> MAFHWCDNNLHTTVFTPRDFQVELLATAYERNTIICLGHRSSKEFIALKLLQELSRRARRHGRVSVYLSCEVGTSTEPCSIYTMLTHLTDLRVWQEQPDMQIPFDHCWTDYHVSILRPEGFLYLLETRELLLSRVELIVLEDCHDSAVYQRIRPLFENHIMPAPPADRPRILGLAGPLHSAGCELQQLSAMLATLEQSVLCQIESASDIVTVLRYCSRPHEYIVQCAPFEMDELSLVLADVLNTHKSFLLDHRYDPYEIYGTDQFMDELKDIPDPKVDPLNVINSLLVVLHEMGPWCTQRAAHHFYQCNEKLKVKTPHERHYLLYCLVSTALIQLYSLCEHAFHRHLGSGSDSRQTIERYSSPKVRRLLQTLRCFKPEEVHTQADGLRRMRHQVDQADFNRLSHTLESKCRMVDQLDQPPTETRALVATLEQILHTTEDRQTNRSAARVTPTPTPAHAKPKPSSGANTAQPRTRRRVYTRRHHRDHNDGSDTLCALIYCNQNHTARVLFELLAEISRRDPDLKFLRCQYTTDRVADPTTEPKEAEL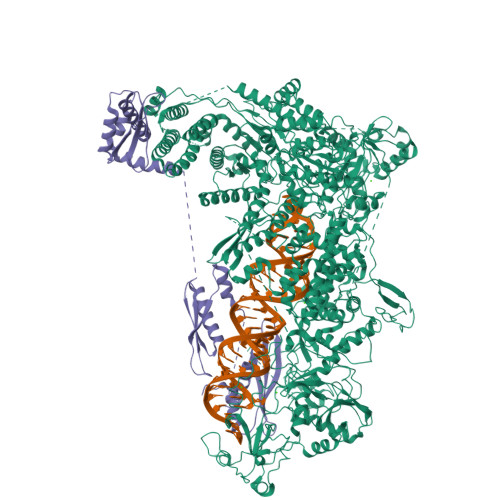EHRRQEEVLKRFRMHDCNVLIGTSVLEEGIDVPKCNLVVRWDPPTTYRSYVQCKGRARAAPAYHVILVAPSYKSPTVGSVQLTDRSHRYICATGDTTEADSDSDDSAMPNSSGSDPYTFGTARGTVKILNPEVFSKQPPTACDIKLQEIQDELPASAQLDTSNSSDEAVSMSNTSPSESSTEQKSRRFQCELSSLTEPEDTSDTTAEIDTAHSLASTTKDLVHQMAQYREIEQMLLSKCANTEPPEQEQCEAERFSACLAAYRPKPHLLTGASVDLGSAIALVNKYCARLPSDTFTKLTALWRCTRNERAGVTLFQYTLRLPINSPLKHDIVGLPMPTQTLARRLAALQACVELHRIGELDDQLQPIGKEGFRALEPDWECFELEPEDEQIVQLSDEPRPGTTKRRQYYYKRIASEFCDCRPVAGAPCYLYFIQLTLQCPIPEEQNTRGRKIYPPEDAQQGFGILTTKRIPKLSAFSIFTRSGEVKVSLELAKERVILTSEQIVCINGFLNYTFTNVLRLQKFLMLFDPDSTENCVFIVPTVKAPAGGKHIDWQFLELIQANGNTMPRAVPDEERQAQPFDPQRFQDAVVMPWYRNQDQPQYFYVAEICPHLSPLSCFPGDNYRTFKHYYLVKYGLTIQNTSQPLLDVDHTSARLNFLTPRYVNRKGVALPTSSEETKRAKRENLEQKQILVPELCTVHPFPASLWRTAVCLPCILYRINGLLLADDIRKQVSADLGLGRQQIEDEDFEWPMLDFGWSLSEVLKKSRESKQKESLKDDTINGKDLVDVEKKAISEETQIDKDSKDDKVEKSAIELIIEGEEKLQEADDFIEIGTWSNDMADDIASFNQEDDDEDDAFHLPVLPANVKFCDQQTRYGSPTFWDVSNGESGFKGPKSSQNKQGGKGKAKGPAKPTFNYYDSDNSLGSSYDDDDNAGPLNYMHHNYSSDDDDVADDIDAGRIAFTSKNEAETIETAQEVEKRQKQLSIIQATNANERQYQQTKNLLIGFNFKHEDQKEPATIRYEESIAKLKTEIESGGMLVPHDQQLVLKRSDAAEAQVAKVSMMELLKQLLPYVNEDVLAKKLGDRRELLLSDLVELNADWVARHEQETYNVMGCGDSFDNYNDHHRLNLDEKQLKLQYERIEIEPPTSTKAITSAILPAGFSFDRQPDLVGHPGPSPSIILQALTMSNANDGINLERLETIGDSFLKYAITTYLYITYENVHEGKLSHLRSKQVANLNLYRLGRRKRLGEYMIATKFEPHDNWLPPCYYVPKELEKALIEAKIPTHHWKLADLLDIKNLSSVQICEMVREKADALGLEQNGGAQNGQLDDSNDSCNDFSCFIPYNLVSQHSIPDKSIADCVEALIGAYLIECGPRGALLFMAWLGVRVLPITRQLDGGNQEQRIPGSTKPNAENVVTVYGAWPTPRSPLLHFAPNATEELDQLLSGFEEFEESLGYKFRDRSYLLQAMTHASYTPNRLTDCYQRLEFLGDAVLDYLITRHLYEDPRQHSPGALTDLRSALVNNTIFASLAVRHGFHKFFRHLSPGLNDVIDRFVRIQQENGHCISEEYYLLSEEECDDAEDVEVPKALGDVFESIAGAIFLDSNMSLDVVWHVYSNMMSPEIEQFSNSVPKSPIRELLELEPETAKFGKPEKLADGRRVRVTVDVFCKGTFRGIGRNYRIAKCTAAKCALRQLKKQGLIAKKD;> MDQENFHGSSLPQQLQNLHIQPQQASPNPVQTGFAPRRHYNNLVGLGNGNAVSGSPVKGAPLGQRHVKLKKEKISAQVAQLSQPGQLQLSDVGDPALAGGSGLQGGVGLMGVILPSDEALKFVSETDANGLAMKTPVSILQELLSRRGITPGYELVQIEGAIHEPTFRFRVSFKDKDTPFTAMGAGRSKKEAKHAAARALIDKLIGAQLPESPSSSAGPSVTGLTVAGSGGDGNANATGGGDASDKTVGNPIGWLQEMCMQRRWPPPSYETETEVGLPHERLFTIACSILNYREMGKGKSKKIAKRLAAHRMWMRLQETPIDSGKISDSICGELEGEPRSSENYYGELKDISVPTLTTQHSNKVSQFHKTLKNATGKKLLKLQKTCLKNNKIDYIKLLGEIATENQFEVTYVDIEEKTFSGQFQCLVQLSTLPVGVCHGSGPTAADAQRHAAQNALEYLKIMTKK Cysteine protease inhibitors (CPI; cystatins) from nematodes have been found to play major roles in modulating host immunity. Cystatins are a group of cysteine protease inhibitors that bind reversibly to cysteine proteases and regulate their proteolytic activities. The predominant target proteases for cystatin are C1 (papain-like cysteine peptidase) and C13 family (legumain). Structurally, a typical cystatin fold contains a five-stranded anti-parallel β-sheet wrapped around an α-helix.

The human gastrointestinal nematode Ascaris lumbricoides infects as many as 1.5 billion people globally and causes malnutrition, retarded growth, reduced physical fitness and reduced work capacity in infected individuals. Although CPIs from many nematode species have been studied extensively for their roles in the induction of immunosuppression, the structural features of this group of immunomodulatory proteins remain largely unknown. In this study, we found that the recombinant Al-CPI strongly inhibited the proteolytic activity of cathepsins. We then analyzed the structure of A. lumbricoides CPI (Al-CPI). We identified the critical segments of Al-CPI molecule that could be involved in the interaction between Al-CPI and its target proteases. Mutagenesis study further confirmed that these segments were responsible for the inhibition of cysteine protease activities.

>[4x]GQVGVPGGFSTKDVNDPKIQALAGKALQRINAASNDLFQQTIVKVISAKTQVVAGTNTVLELLIAPTSCRKNETSAGNCEAVSNGTKQICTVAIWEKPWENFEEITIKECKSA> SYDQAFLEQYEKIKDPASGYFREFNGLLVPYHSVETMIVEAPDHGHQTTSEAFSYYLWLEAYYGRVTGDWKPLHDAWESMETFIIPGTKDQPTNSAYNPNSPATYIPEQPNADGYPSPLMNNVPVGQDPLAQELSSTYGTNEIYGMHWLLDVDNVYGFGFCGDGTDDAPAYINTYQRGARESVWETIPHPSCDDFTHGGPNGYLDLFTDDQNYAKQWRYTNAPNADARAVQVMFWAHEWAKEQGKENEIAGLMDKASKMGDYLRYAMFDKYFKKIGNCVGATSCPGGQGKDSAHYLLSWYYSWGGSLDTSSAWAWRIGSSSSHQGYQN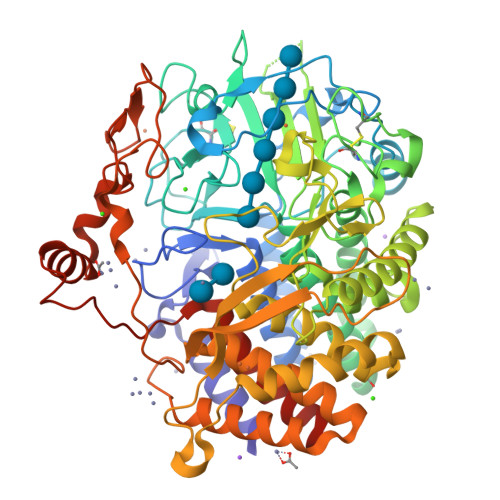VLAAYALSQVPELQPDSPTGVQDWATSFDRQLEFLQWLQSAEGGIAGGATNSWKGSYDTPPTGLSQFYGMYYDWQPVWNDPPSNNWFGFQVWNMERVAQLYYVTGDARAEAILDKWVPWAIQHTDVDADNGGQNFQVPSDLEWSGQPDTWTGTYTGNPNLHVQVVSYSQDVGVTAALAKTLMYYAKRSGDTTALATAEGLLDALLAHRDSIGIATPEQPSWDRLDDPWDGSEGLYVPPGWSGTMPNGDRIEPGATFLSIRSFYKNDPLWPQVEAHLNDPQNVPAPIVERHRFWAQVEIATAFAAHDELFGAGAP> MSKSKVDNQFYSVEVGDSTFTVLKRYQNLKPIGSGAQGIVCAAYDAVLDRNVAIKKLSRPFQNQTHAKRAYRELVLMKCVNHKNIISLLNVFTPQKTLEEFQDVYLVMELMDANLCQVIQMELDHERMSYLLYQMLCGIKHLHSAGIIHRDLKPSNIVVKSDCTLKILDFGLARTAGTSFMMTPYVVTRYYRAPEVILGMGYKENVDIWSVGCIMGEM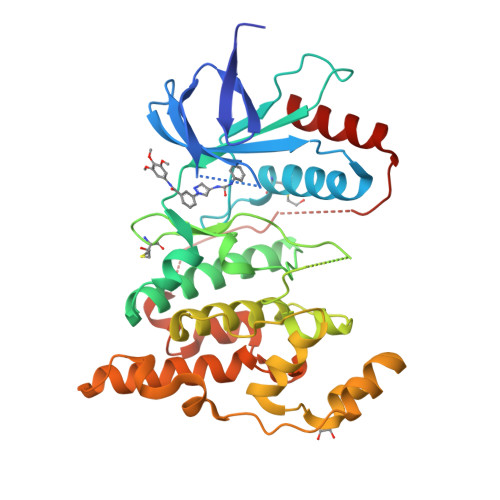VRHKILFPGRDYIDQWNKVIEQLGTPCPEFMKKLQPTVRNYVENRPKYAGLTFPKLFPDSLFPADSEHNKLKASQARDLLSKMLVIDPAKRISVDDALQHPYINVWYXXXXXXDEREHTIEEWKELIYKEVMNSE HGbRL from M. infernorum is a putative globin-coupled sensor of 274 residues, consisting of an N-terminal globin domain and a C-terminal Roadblock/LC7 domain. N-HGbRL consists of seven α-helices, helices A–H, lacks helix D and forms a dimer. It displays a typical bacterial globin fold except for a very untypical feature — its helices E and F unexpectedly fuse into an elongated helix. In other words, both the proximal and distal sites of a single globin fold are constituted mainly by two separate subunits, representing the first ever site-swapping example in the globin family.

The structure of N-HGbRL was first solved in the open form in space group C2, with two subunits in the asymmetric unit. In the distal site, an imidazole molecule from the Ni2+-affinity chromatography binds to the haem and the highly conserved Tyr28(B10), which also coordinates a water molecule, W1. The distal site of N-HGbRL is lined by all hydrophobic residues (Phe27, Leu31, Phe42, Leu53, Val56, Val94 and Leu98) except for Tyr28(B10) and Lys52(E10). The A-ring propionate of the haem also hydrogen-bonds to the side chains of Arg80 and Tyr84, and the D-ring propionate to Lys43 N and the Tyr28-bound water W1. A ~ 25° bending of helix E results in a large shift of subunits B* between the two forms, creating a huge pocket of about 250 Å3 in the distal site of the open form that connects to several tunnels. The huge pocket of N-HGbRL’s open structure may be able to bind a comparatively large ligand. In the open form, interaction between subunits B* from two adjacent asymmetric units, Arg39(C5) from one asymmetric unit and Glu47 from the other, causes loop CE to shift relative to that of subunit A*. When comparing their highly conserved Gln(E7)–Leu(E15) regions, however, helix E of N-HGbRL’s open form is moved forwards by about a helical turn relative to that of HGbI, leading to a structural ‘frameshift’ of three residues. HGbI also has a smaller distal pocket which is connected to the solvent through several tunnels, but the distal pocket of the open form of N-HGbRL is readily accessible from the solvent through an opening. When a signalling ligand binds the haem in the closed form, it dislodges Lys52(E10) and pushes helix E outwards, inducing part of loop CE to fold into the extra turn of helix E of the open form.

>MTREEIKMIQKSWLRVIDKMDEAGLLFYRRLFDVEPKVRPLFKIDIEKQGRKLMDVLNWIVLNLQDIDAALDAARELARRHVKYGVKAEHYPVVGHTLIWTLRKMIGSEWTKQLEQLWTQAYEALAQVMIEEHHHHHH[2x]2-fluoro-N,3-dimethylbenzene-1-sulfonamide | C8 H10 F N O2 S | 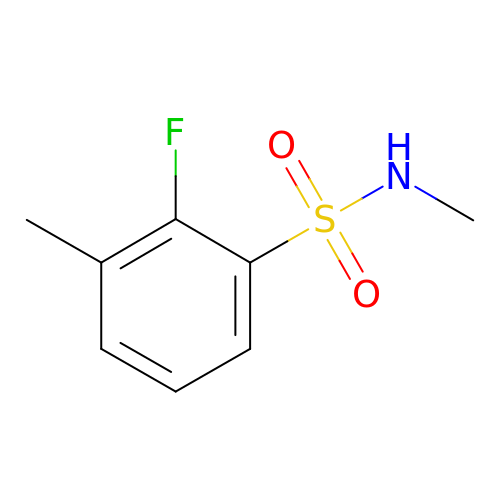PXJRMCHXJXWNJG-UHFFFAOYSA-N>[2x]ARTEKIYIYGASGHGLVCEDVAKNMGYKECIF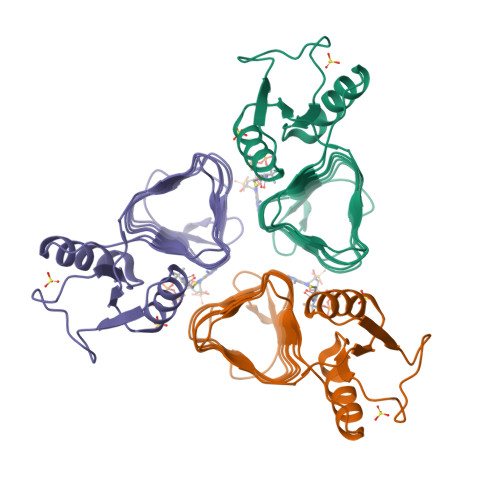LDDFKGMKFESTLPKYDFFIAIGNNEIRKKIYQKISENGFKIVNLIHKSALISPSAIVEENAGILIMPYVVINAKAKIEKGVILNTSSVIEHECVIGEFSHVSVGAKCAGNVKIGKNCFLGINSCVLPNLSLADDSILGGGATLVKNQDEKGVFVGVPAKRM> MHHHHHHMNVKVPMHGQCSFHAELQQKGKNFDMFAVPYQQDPALALKEFRAQLPIFFSEAMGYWIVTRYEDVKAIFRDPITFSACNALEKLTPSCPEALKILEKYKYGMNRTLVNEDEPVHMERRRALMDAFTPQNLEEHQHFVRELVRKKVDGFIYKGRADLVQEMLWEIPLMVALHFLGVPEDDMQELRKFAVAH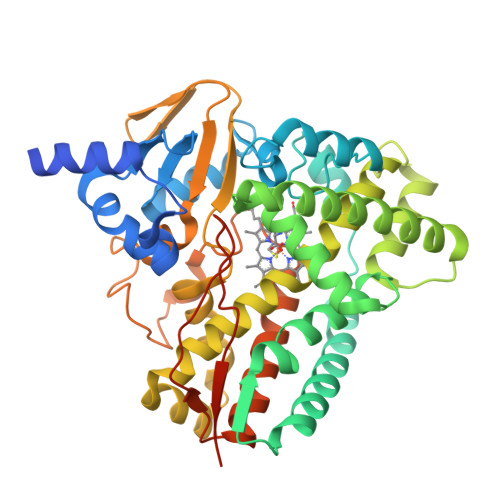TVNTWGRPTLEQQLEVAEGVGQFWEYSGRVLEKMKNNPEGKGWMYDMIAKNRVMPEVVTDNYLHSMMMAIMVAAHETTALASANALKLLLADRKVWKKICDNPQLIPGAVEECLRHSGSVVAWRRQVTTESEVSGVKFRKGDKLFLVSASANHDELHFENADELDIYRDNAIEHLTFGYGAHQCMGKNIGRMEMCIFIEELSRRIPDLKLCEQEFTYLANTSFRGPEALWTEWQAQPEQTARQITSFPIGAP> MRSSILFLLKLMKIMDVQQQQEAMSSEDRFQELVDSLKPRTAHQYKTYYTKYIQWCQLNQIIPTPEDNSVNSVPYKDLPISAELIHWFLLDTLITDDKPGEKREETEDLDEEEENSFKIATLKKIIGSLNFLSKLCKVHENPNANIDTKYLESVTKLHTHWIDSQKAITTNETNNTNTQVLCPPLLKVSLNLWNPETNHLSEKFFKTCSEKLRFLVDFQLRSYLNLSFEERSKIRFGSLKLGKRDRDAIIYHKVTHSAEKKDTPGHHQLLALLPQDCPFICPQTTLAAYLYLRFYGIPSVSKGDGFPNLNADENGSLLQDIPILRGKSLTTYPREETFSNYYTTVFRYCHLPYKRREYFNKCNLVYPTWDEDTFRTFFNEENHGNWLEQPEAFAFPDKIPFDFKKIMNFKSPYTSYSTNAKKDPFPPPKDLLVQIFPEIDEYKRHDYEGLSQNSRDFLDLMEVLRERFLSNLPWIYKFFPNHDIFQDPIFGNSDFQSYFNDKTIHSKGSPILSFDILPGFNKIYKNKTNFYSLLIERPSQLTFASSHNPDTHPTQKQESEGPLQMSQLDTTQLNELL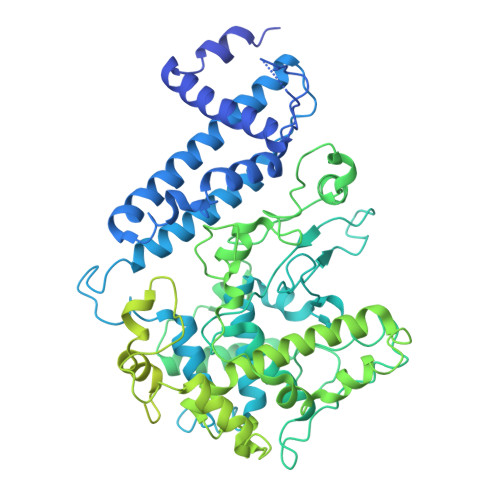KQQSFEYVQFQTLSNFQILLSVFNKIFEKLEMKKSSRGYILHQLNLFKITLDERIKKSKIDDADKFIRDNQPIKKEENIVNEDGPNTSRRTKRPKQIRLLSIADSSDESSTEDSNVFKKDGESIEDGAYGENEDENDSEMQEQLKSMINELINSKISTFLRDQMDQFELKINALLDKILEEKVTRIIEQKLGSHTGKFSTLKRPQLYMTEEHNVGFDMEVPKKLRTSGKYAETVKDNDDHQAMSTTASPSPEQDQEAKSYTDEQEFMLDKSIDSIEGIILEWFTPNAKYANQCVHSMNKSGNKSWRANCEALYKERKSIVEFYIYLVNHESLDRYKAVDICEKLRDQNEGSFSRLAKFLRKWRHDHQNSFDGLLVYLSN> MNLILLGPPGAGKGTQAEKIVEEYGIPHISTGDMFRAAIKEGTELGLKAKEYMDKGELVPDEVTIGLVKERLSQPDCKKGFLLDGFPRTVAQAEALDKILKELGIKLDAVINIEVPREELLERLTGRRVCRQCGATYHVIFNPPKVEGVCDKCGGELYQRSDDNEETVSNRLDVYEDQTAPLIDYYEKKGLLKNIDGDQDIDA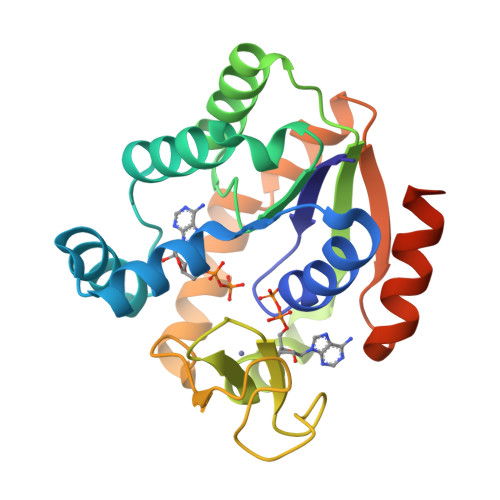VFADIKAALGRDKQGGGENLYFQ> C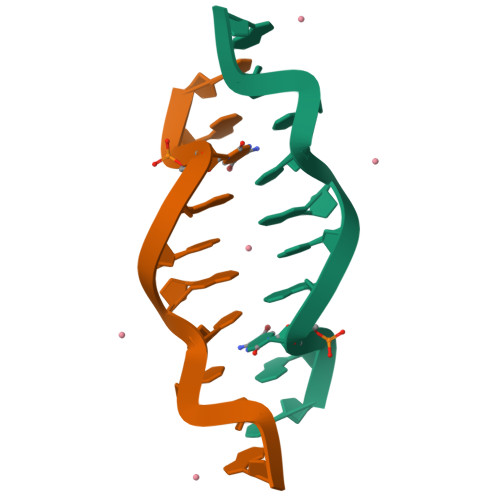GCGGGCGCG> SQEVMKNLSLNFGKALDECKKEMTLTDAINEDFYNFWKEGYEIKNRETGCAIMCLSTKLNMLDPEGNLHHGNAMEFAKKHGADETMAQQLIDIVHGCEKSTPANDD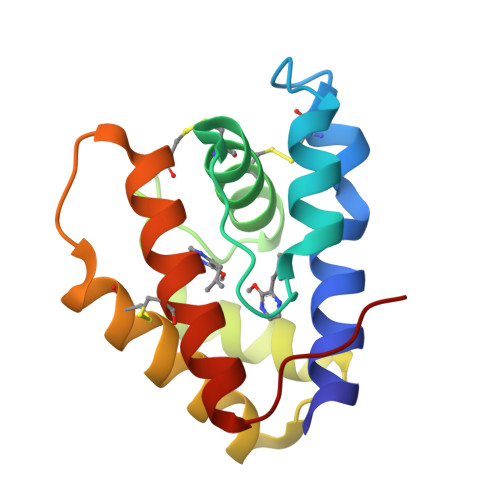KCIWTLGVATCFKAEIHKLNWAPSMD> MAGWNAYIDNLMADGTCQDAAIVGYKDSPSVWAAVPGKTFVNITPAEVGV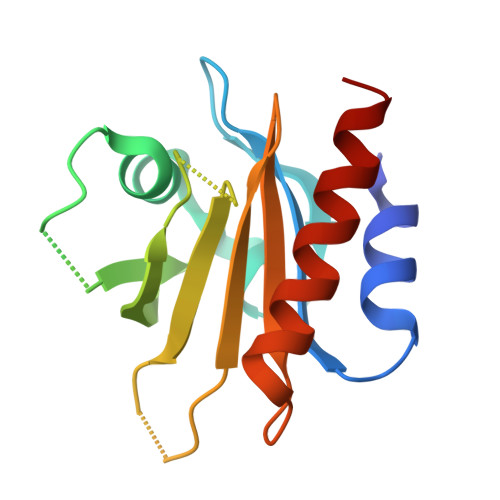LVGKDRSSFYVNGLTLGGQKCSVIRDSLLQDGEFSMDLRTKSTGGAPTFNVTVTKTDKTLVLLMGKGGVHGGLINKKCYEMASHLRRSQY> TAHRFLFVSTPVGPLGSGRGGGVELTLPNLAKALTQRGHQVSVLAPAGSVLPDLPLETVPGTWQSTAQSHGRATPAEIPAESVLARLWDRAHQQQADFDLILNFAYDWLPLYLTPFFKTPVAHLISMGSLSEVMDQAIATSLDRYPGSIAVHSLAQAATFPFGDRCLCIGNALDLAAYGFNPEPEPVLGWVGRIAPEKGLEDAIQAAQQAGLPLRVWGALTEPDYWQRLQQQFGDRAVS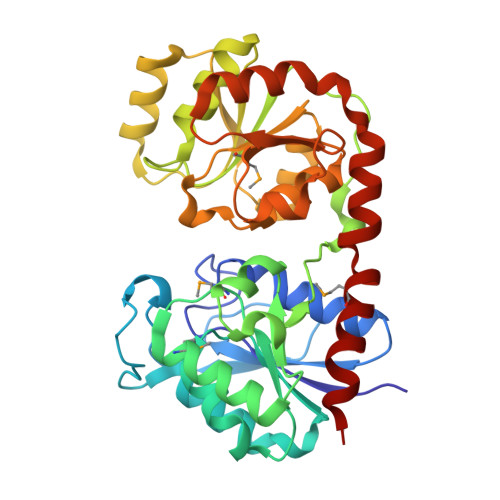YQGFVSTDELQRGLGRCQGLLMTPKWVEAFGNVAIEALACGLPVIAYARGGPLEIIEQGKSGWLVEPDQQAALVNAIGQLSSLDRAYCRAQAEARFSLAAMGQRLEAWLLPLLS>[2x]QVT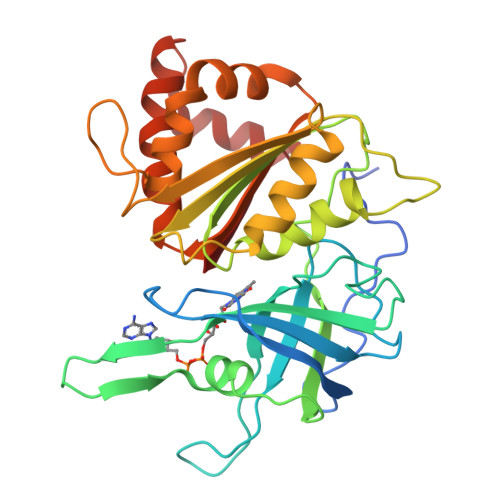TEAPAKVVKHSKKQDENIVVNKFKPKEPYVGRCLLNTKITGDDAPGETWHMVFSTEGEVPYREGQSIGIVPDGIDKNGKPHKLRLYSIASSAIGDFGDSKTVSLCVKRLVYTNDAGEVVKGVCSNFLCDLKPGSEVKITGPVGKEMLMPKDPNATVIMLGTGTGIAPFRSFLWKMFFEKHEDYQFNGLAWLFLGVPTSSSLLYKEEFEKMKEKAPENFRLDFAVSREQVNDKGEKMYIQTRMAQYAEELWELLKKDNTFVYMMGLKGMEKGIDDIMVSLAAKDGIDWIEYKRTLKKAEQWNVEVY> MDNPNPGPDGEGEVELEKDSNVVLTTQRDPSTSIPAPVSVKWSRWTSNDVVDDYATITSRWYQIAEFVWSKDDPFDKELARLILPRALLSSIEANSDAICDVPNTIPFKVHAYWRGDMEVRVQINSNKFQVGQLQATWYYSDHENLNISSKRSVYGFSQMD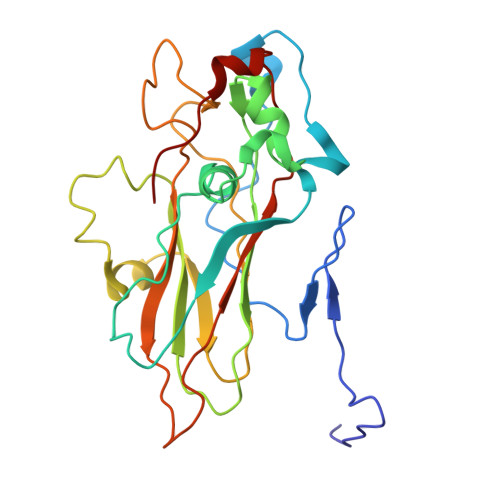HALISASASNEAKLVIPFKHVYPFLPTRIVPDWTTGILDMGALNIRVIAPLRMSATGPTTCNVVVFIKLNNSEFTGTSSGKFYASQIRA The earlier discovery of the pathway responsible for alkane biosynthesis in cyanobacteria allowed the conversion from solar energy to alkanes through photosynthesis, without providing external carbon sources. This two-step pathway utilizes two water-soluble enzymes, namely acyl-acyl carrier protein (acyl-ACP) reductase (AAR) and aldehyde-deformylating oxygenase (ADO). AAR catalyzes the first step of this pathway, reducing the substrate fatty acyl-ACP/fatty acyl-coenzyme A (acyl-CoA) into the corresponding aldehyde in a NADPH-dependent manner. Subsequently, ADO catalyzes the conversion of fatty aldehyde into alk(a/e)ne with one carbon shorter (Cn-1 hydrocarbon) and the formate as a C1-derived form. Here we report the crystal structure of AAR from Synechococcus elongatus PCC 7942 (SeAAR) in its apo form (AARapo), together with three structures of AAR in complex with ADO from the same species of cyanobacteria (SeADO), in which AAR binds either substrate or substrate/cofactor.

In our AARthioester–ADO structure solved at 2.18 Å resolution, we observed a long tube-shaped electron density, which can be well fitted with a stearic chain, within an interior tunnel of AAR. No electron density corresponding to the CoA moiety was observed, despite the incubation of stearoyl-CoA with AAR prior to crystallization. This finding indicates that the acyl-enzyme intermediate was spontaneously formed, and the CoA moiety had already been released. The structure showed that the C1 atom of the stearoyl chain (stearoyl-C1) had formed a covalent thioester bond with the hydrosulfide group of C294 (C294-SH). Mass spectrometric analysis of the stearoyl-CoA-incubated AAR sample that was used for crystallization confirmed the thioester bond formation, thus the AARthioester–ADO structure represents the acyl-enzyme intermediate state of AAR. In the AARthioester–ADO structure, the stearic chain is buried inside a hydrophobic tunnel (acyl-tunnel) formed mainly by non-polar residues from the NTD and CTD of AAR. One end of the acyl-tunnel connects with the wide cleft above C294, forming an L-shaped, long channel. At the other end, the acyl-tunnel can be seen to extend toward the AAR–ADO interface with its opening surrounded by residues Y23 and Y26 from the NTD of AAR and sealed by M221 of ADO. In the AARapo structure, this acyl-tunnel is broken by the side chains of M279 and M21. Both M279 and M21 undergo significant conformational changes in the AARthioester–ADO structure, where they participate in forming the acyl-tunnel. While helix 7 of ADO interacts with the NTD of AAR, the acidic residues of this helix form strong electrostatic interactions with the basic residues from the long helical region (R73–H91), as well as R118 from Fr-II of AAR.

> MFGLIGHLTSLEQARDVSRRMGYDEYADQGLEFWSSAPPQIVDEITVTSATGKVIHGRYIESCFLPEMLAARRFKTATRKVLNAMSHAQKHGIDISALGGFTSIIFENFDLASLRQVRDTTLEFERFTTGNTHTAYVICRQVEAAAKTLGIDITQATVAVVGATGDIGSAVCRWLDLKLGVGDLILTARNQERLDNLQAELGRGKILPLEAALPEADFIVWVASMPQGVVIDPATLKQPCVLIDGGYPKNLGSKVQGEGIYVLNGGVVEHCFDIDWQIMSAAEMARPERQMFACFAEAMLLEFEGWHTNFSWGRNQITIEKMEAIGEASVRHGFQPLALAI;> MRTPWDPPNPTFSLSSVSGDRRLMPQLEASLELDFQSESYKDAYSRINAIVIEGEQEAFDNYNRLAEMLPDQRDELHKLAKMEQRHMKGFMACGKNLSVTPDMGFAQKFFERLHENFKAAAAEGKVVTCLLIQSLIIECFAIAAYNIYIPVADAFARKITEGVVRDEYLHRNFGEEWLKANFDASKAELEEANRQNLPLVWLMLNEVADDARELGMERESLVEDFMIAYGEALENIGFTTREIMRMSAYGLAAV>GSMGTVPPSREDRNRSQLWPIRMDRLEGQRVCTAGGRYIVELDTRCRFEVAAQGNFVKRILIVEVDEMVQTVYVHRIPDRTVRGRNGEEELITLTNNPFVYTSYSQMPKEVQNDYMRLQKMVAVTISGRVAKVTFRRPSQFPDAQAQLMENGDLRIKLPRSVIVRKMDNG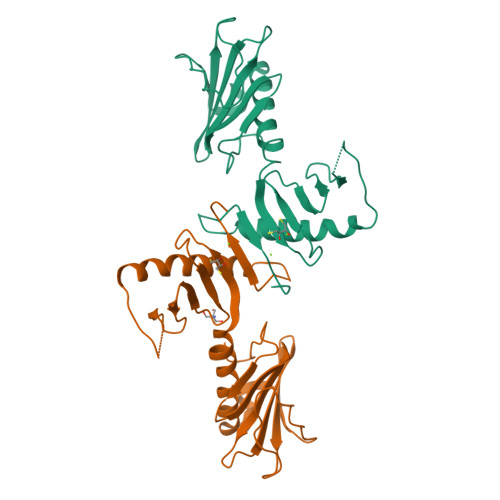EIFNCIDGIATQKQAVSGITLTKVNEVYKYLIRFEQCLNGMDRGMVCFPIVFSAGTNMVG[2x]> MRNRGFGRRELLVAMSMLVSVTGCARHASGARPASTTLPAGADLADRFAELERRYDARLGVYVPATGTTAAIEYRADERFAFCSTFKAPLVAAVLHQNPLTHLDKLITYTSDDIRSISPVAQQHVQTGMTIGQLCDAAIRYSDGTAANLLLADLGGPGGGTAAFTGYLRSLGDTVSRLDAEEPELNRDPPGDERDTTTPHAIALVLQQLVLGNALPPDKRALLTDWMARNTTGAKRIRAGFPADWKVIDKTGTGDYGRANDIAVVWSPTGVPYVVAVMSDRAGGGYDAEPREALLAEAATCVAGVLA

BlaC is a class A β-lactamase and due to its broad substrate specificity towards β-lactams, β-lactam antibiotics alone are not an efficacious treatment course for TB infections. BlaC, a hydrolase (EC 3.5.2.6), cleaves lactam carbon–nitrogen amide bonds rapidly, effectively deactivating β-lactam antibiotics. As previously reported for BlaC and other class A serine β-lactamases such as TEM-1, SHV-1, and the CTXMs, the global fold consists of two domains, the α-domain and the α/β-domain. Located in the α-domain, adjacent to the α/β-domain, are the catalytic residues Ser-70, Lys-73 and Glu-166 (numbered according to Ambler notation).

Herein, we provide crystal structure evidence to demonstrate that the serine β-lactamase BlaC can be phosphorylated at its nucleophilic serine by the novel β-lactamase inhibitors based on a bis(benzoyl) phosphate scaffold. In the case of the phosphoserine crystal, Ser-70 showed clear density for a phosphoserine having been phosphorylated by the inhibitor bis(benzoyl) phosphate. The phosphoserine structure resolved to 1.52 Å. The phosphoserine crystal was in the P212121 space group. Additionally, the phosphoserine BlaC structure contained phosphate molecules near the active site adjacent to the nucleophilic Ser-70. In the phosphoserine structure, the distance between the oxygen atom of the phosphorylated Ser-70 and the phosphorus atom of the closest phosphate molecule was 4.5 Å (phosphate pictured above Ser-70 in Figure 3B). In addition, even though the previously published BlaC structures contain phosphate molecules near the active site, they do not have a phosphorylated Ser-70. Consistent with the proposed phosphorylation mechanism, we did not observe an intact inhibitor, nor released benzoates in the active site after the phosphorylation step occurred. A plausible reason why the bis(benzoyl) phosphate scaffold worked over other organophosphate scaffolds might involve the electrophilic nature of the phosphorus center and the pKa of the leaving groups’ conjugate acids (e.g., benzoic acids vs. alcohols and thiols). This new crystal-structure evidence suggests the inactivation mechanism of BlaC involves the unsubstituted bis(benzoyl) phosphate via nucleophilic Ser-70 phosphorylation, and is expected to aid in the design of future novel β-lactamase inactivators utilizing a phosphorylating scaffold.> 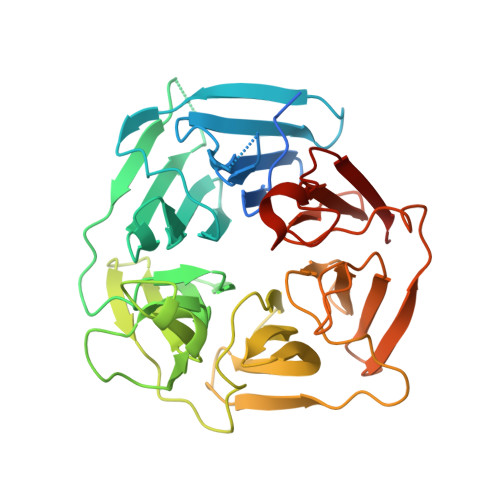GADGNEDLRADDLPGPAFESYESMELACPAERSGHVAVSDGRHMFVWGGYKSNQVRGLYDFYLPREELWIYNMETGRWKKINTEGDVPPSMSGSCAVCVDRVLYLFGGHHSRGNTNKFYMLDSRSTDRVLQWERIDCQGIPPSSKDKLGVWVYKNKLIFFGGYGYLPEDKVLGTFEFDETSFWNSSHPRGWNDHVHILDTETFTWSQPITTGKAPSPRAAHACATVGNRGFVFGGRYRDARMNDLHYLNLDTWEWNELIPQGICPVGRSWHSLTPVSSDHLFLFGGFTTDKQPLSDAWTYCISKNEWIQFNHPYTEKPRLWHTACASDEGEVIVFGGCANNLLVHHRAAHSNEILIFSVQPK> MTTPISPPPQWSRRRQEKQRRLERVRGLADGAVLPREGLVAALEALIAPGDRVVLEGNNQKQADFLSRSLARVDPGKLHDLHMIMPSVGRPEHLDLFELGIARKLDFSFSGPQSLRIGQLLEDGLLEIGAIHTYIELYARLVVDLIPNVALVAGFVADREGNVYTGPSTEDTPALVEPTAFSDGIVIVQVNRIVDDPRDLPRVDIPASWVDFVVEADQPFYIEPLFTRDPRHIKPVHVLMAMMAIRGIYQRHNVQSLNHGIGFNTAAIELILPTYGESLGLKGKICRHWTLNPHPTLIPAIESGWVESVHCFGTELGMEGYIAQRPDVFFTGRDGSLRSNRMFCQLAGQYAVDLFIGATLQVDGDGHSSTVTRGRLAGFGGAPNMGHDPRGRRHSTPAWLDMRGEPEA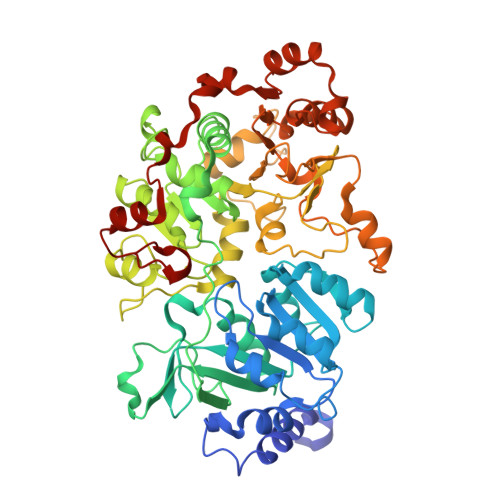LLERGRKLVVQMVETFQDGGKPTFVERLDALEVARQTGMPLAPVMIYGDDVTHVLTEEGIAYLYKARSLEERQAMIAAVAGISPIGLRHDPRETQRMRREGLIALPEDLGIRRTDASRELLAAKSIAELVEWSGGLYQPPARFRSW> MRTTKKIVSAVLAACMLASTAVVSSFAATADDSSAVSSDYARDNSYTKAAEDIDAQYAYSGNDLGVTYTKDATTFKVWSPTATGVKLNIFTKGSDDEQGASKVASYTLEKMLVDGEWNGVWTITLVGEWKDYYYTYSVTTTDTTHIGSDATKTYETQDVYSTATGVNGKRSMIVDLDETDPEGWSNDSHVLLDKSTKSSVWELHIKDFSYDKASGVSDANRGKYLAFTENGTTLNGEGKVSTCIDYLKELGVTTVQLNPFYDFQSVNEAGDDSQFNWGYDPVNYNVPEGSYSSNPYDGKVRIKECKEMIKALHDAGISVVMDVVYNHTYSTDSCFQYTVPNYYYRMKTTGAFSDGSGCGNEGATERAMYRQYVIDSLKYWVNEYHVDGFRFALMGLMDVETMNMAREALDQIDPRITMWGEGWAGGDSYHPTNTCSGTKFYPATQANASRLSDRIAIFNDGIRDGIKGSAMDISDVGFIQGSKSSAKGVSYGVRANSSGTYKWKAQAPSQCVTYDACHDNATLYDQIIA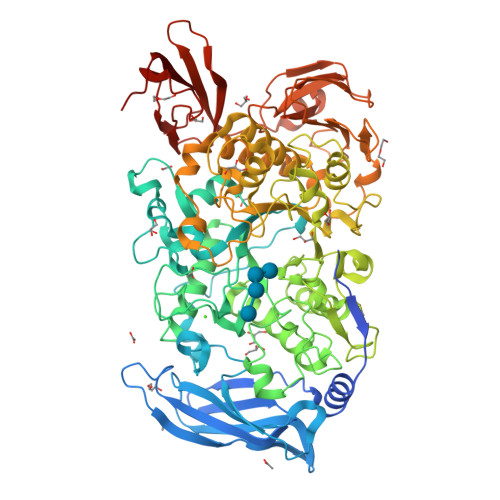STGLADYGERNSEAVKMNRLASAIIYTSQGISFTLAGEEMARSKDGDTNSYKSAANLNMIKWQNVVDYADVVSYYKGMMQIKSAFSPLTAMDNSYADKYTFTKKVSASTNQISFTIQNDVEGEWNKMAVIYNNATTAADVTLSDTSVTDWVVIANGETAGLDSLGEVTGSTFTVPARSAIVAVDKAGYESAGIHSSKGKVKVNYVYEATGEKLEDSVILQGSVGSGYVTVPSAVIPDTYIVSRIGGNAEGKYTSDMQEVTYYYTDYIPES The Lon protease is a AAA+ protein found in prokaryotes, archaea, and eukaryotic organelles. Lon is involved in cellular protein homeostasis by degrading damaged or misfolded abnormal proteins, which prevents these unwanted protein species from forming toxic aggregates. Lon is known to form a homohexamer; each protomer is composed of multiple domains, including an N-terminal substrate-binding globular domain (NGD), a long-helix domain (LH), a three-helix bundle (3H), a AAA+ ATPase module, and a protease domain. We show here, using cryo-electron microscopy (cryo-EM), that the activation process of the Lon AAA+ protease may involve a pentameric assembly and a substrate-dependent incorporation of the sixth protomer to form the substrate-pore-loop contacts seen in the translocating state.

To provide a comparative context, we also examined wild-type MtaLon in two states: without any nucleotide (MtaLon-Apo) and incubated with 5 mM ADP (MtaLon:ADP). Unexpectedly, both MtaLon-Y224S:ATPγS and wild-type MtaLon, whether with ADP or lacking nucleotide, predominantly formed left-handed spiral pentamers or spiral hexamers, rather than closed-ring hexamers. The substrate-free hexameric form also adopts a left-handed spiral structure. It is composed of the tethered pentamer and an additional Ac-protomer, Ac6*, which binds next to the protomer Ob1 and occupies the lowermost position of the spiral. Interestingly, the 3H subdomain of Ac6* occupies the axial cavity of the spiral complex and binds to the ATPase domains of the protomers 1–5, effectively blocking the accessibility of the pore loops and forming an inactive structure.

>MRLELPVIPLRNTVILPHTTTPVDVGRAKSKRAVEEAMGADRLIFLVAQRDPEVDDPAPDDLYTWGVQAVVKQAMRLPDGTLQVMVEARARAQVTDYIPGPYLRARGEVFSEIFPIDEAVVRVLVEELKEAFEKYVANHKSLRLDRYQLEAVKGTSDPAMLADTIAYHATWTVAEKQEILELTDLEARLKKVLGLLSRDLERFELDKRVAQRVKEQMDTNQREYYLREQMKAIQKELGGEDGLSDLEALRKKIEEVGMPEAVKTKALKELDRLERMQQGSPEATVARTYLDWLTEVPWSKADPEVLDINHTRQVLDEDHYGLKDVKERILEYLAVRQLTQGLDVRNKAPILVLVGPPGVGKTSLGRSIARSMNRKFHRISLGGVRDEAEIRGHRRTYIGAMPGKLIHAMKQVGVINPVILLDEIDKMSSDWRGDPASAMLEVLDPEQNNTFTDHYLDVPYDLSKVFFITTANTLQTIPRPLLDRMEVIEIPGYTNMEKQAIARQYLWPKQVRESGMEGRIEVTDAAILRVISEYTREAGVRGLERELGKIARKGAKFWLEGAWEGLRTIDASDIPTYLGIPRYRPDKAETEPQVGTAQGLAWTPVGGTLLTIEVAAVPGSGKLSLTGQLGEVMKESAQAALTYLRAHTQDYGLPEDFYNKVDLHVHVPDGATPKDGPSAGITMATAIASALSRRPARMDIAMTGEVSLRGKVMPIGGVKEKLLAAHQAGIHKIVLPKDNEAQLEELPKEVLEGLEIKLVEDVGEVLEYLLLPEPTMPPVVQPSDNRQQPGAGA[6x]> MSRNGELCLKKVIISYCPSNGAPNTRQFLATHLPHFHAKYPSVSIDLRPRLWPEMAITGVYRDGSERSYNTKNLSPMGIFLRLNNLVSTANDYDQPFCASHLHFQRRSVQG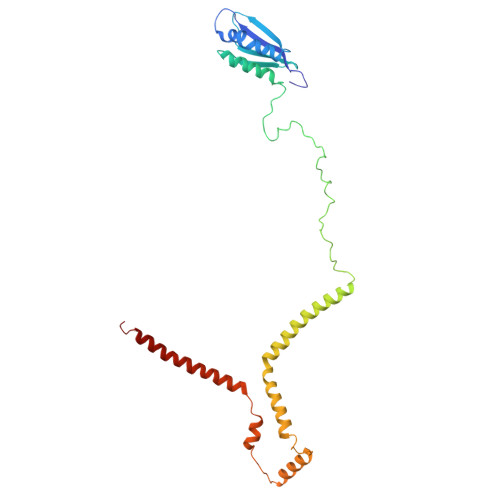TWNPWLWNYETERRRTEAPQWRRKLSEKEWDYYVGQYSAQMKQEEDEIQRRVADRTCVQEQSTREVQERWKRHVVPRMQTDLEFNLSHFKRQHARGQLQQRPVTMGEYRLFSVPDPRELGQDAVDTMRRRESHNMEVWWRKRKEQLKPP1-(5-amino-1,3-dihydro-2H-isoindol-2-yl)ethan-1-one 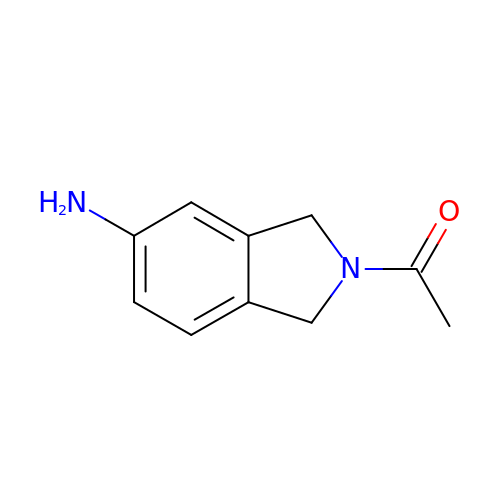| C10 H12 N2 O | YIOYWZUOBVMFGA-UHFFFAOYSA-N>[2x]MSIITDVYAREVLDSRGNPTLEVEVYTESGAFGRGMVPSGASTGEHEAVELRDGDKSRYLGLGTQKAVDNVNNVIADAIIGFDVRDQQAIDRAMIALDGTPNKGKLGANAILGVSIAVARAAADYLEVPLYTYLGGFNTKVLPTPMMNIINGGSHSDAPIAFQEFMILPVGAPSFKEGLRWGAEVFHALKKILKARGLVTAVGDEGGFAPKFEGTEDGVET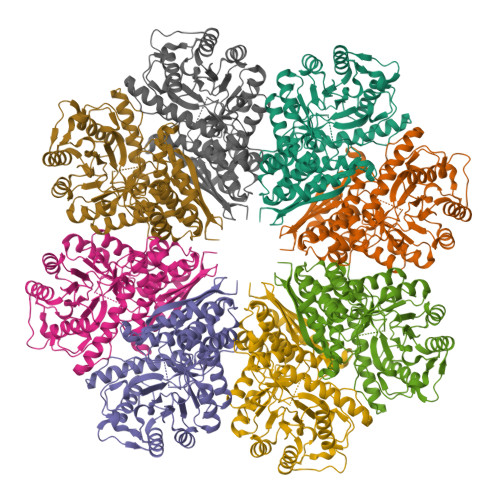IIEAIEAAGYEAGENGIMIGFDCASSEFYDKERKVYDYTKFEGEGAAVRTSAEQIDYLEELVNKYPIITIEDGMDENDWDGWKALTERLGKRVQLVGDDFFVTNTDYLARGIKEGAANSILIKVNQIGTLTETFEAIEMAKEAGYTAVVSHRSGETEDSTIADIAVATNAGQIKTGSLSRTDRIAKYNQLLRIEDQLGEVAVYKGLNSFYNLKKLEHHHHHH>[6x]MKHMPRKMYSCAFETTTKVEDCRVWAYGYMNIEDHSEYKIGNSLDEFM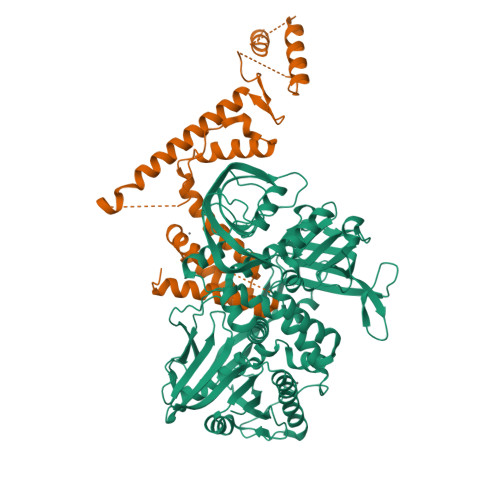AWVLKVQADLYFHNLKFAGAFIINWLERNGFKWSADGLPNTYNTIISRMGQWYMIDICLGYKGKRKIHTVIYDSLKKLPFPVKKIAKDFKLTVLKGDIDYHKERPVGYKITPEEYAYIKNDIQIIAEALLIQFKQGLDRMTAGSDSLKGFKDIITTKKFKKVFPTLSLGLDKEVRYAYRGGFTWLNDRFKEKEIGEGMVFDVNSLYPAQMYSRLLPYGEPIVFEGKYVWDEDYPLHIQHIRCEFELKEGYIPTIQIKRSRFYKGNEYLKSSGGEIADLWLSNVDLELMKEHYDLYNVEYISGLKFKATTGLFKDFIDKWTYIKTTSEGAIKQLAKLMLNSLYGKFASNPDVTGKVPYLKENGALGFRLGEEETKDPVYTPMGVFITAWARYTTITAAQACYDRIIYCDTDSIHLTGTEIPDVIKDIVDPKKLGYWAHESTFKRAKYLRQKTYIQDIYMKEVDGKLVEGSPDDYTDIKFSVKCAGMTDKIKKEVTFENFKVGFSRKMKPKPVQVPGGVVLVDDTFTIK;>XXXXXXXXXXXXXXXXXXXXXXXXXXXXXXXXXXANMRYQFEKNAYGVVASKAKIAEIERNTKEVQRLVDEKIKAMKDKEYYAGGKPQGTIEQRIAMTSPAHVTGINRPHDFDFSKVRSYSRLRTLEESMEMRTDPQYYEKKMIQLQLNFIKSVEGSFNSFDAADELIEELKKIPPDDFYELFLRISEISFEEFDSEGNTVENVEGNVYKILSYLEQYRRGDFDLSLKGF[6x]> MAKKTSSKGKLPPGPSPLPVLGNLLQMDRKGLLRSFLRLREKYGDVFTVYLGSRPVVVLCGT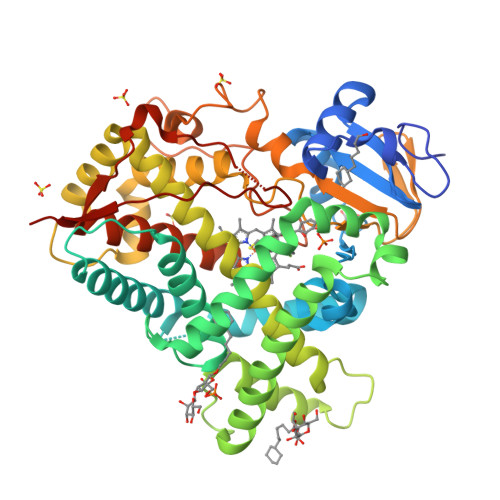DAIREALVDQAEAFSGRGKIAVVDPIFQGYGVIFANGERWRALRRFSLATMRDFGMGKRSVEERIQEEARCLVEELRKSKGALLDNTLLFHSITSNIICSIVFGKRFDYKDPVFLRLLDLFFQSFSLISSFSSQVFELFSGFLKYFPGTHRQIYRNLQEINTFIGQSVEKHRATLDPSNPRDFIDVYLLRMEKDKSDPSSEFHHQNLILTVLSLFFAGTETTSTTLRYGFLLMLKYPHVTERVQKEIEQVIGSHRPPALDDRAKMPYTDAVIHEIQRLGDLIPFGVPHTVTKDTQFRGYVIPKNTEVFPVLSSALHDPRYFETPNTFNPGHFLDANGALKRNEGFMPFSLGKRICLGEGIARTELFLFFTTILQNFSIASPVPPEDIDLTPRESGVGNVPPSYQIRFLARHHHH>[2x]MHNDKDLSTWQTFRRLWPTIAPFKAGLIVAGVALILNAASDTFMLSLLKPLLDDGFGKTDRSVLVWMPLVVIGLMILRGITSYVSSYCISWVSGKVVMTMRRRLFGHMMGMPVSFFDKQSTGTLLSRITYDSEQVASSSSGALITVVREGASIIGLFIMMFYYSWQLSIILIVLAPIVSIAIRVVSKRFRNISKNMQNTMGQVTTSAEQMLKGHKEVLIFGGQEVETKRFDKVSNRMRLQGMKMVSASSISDPIIQLIASLALAFVLYAASFPSVMDSLTAGTITVVFSSMIALMRPLKSLTNVNAQFQRGMAACQTLFTILDSEQEKDEGKR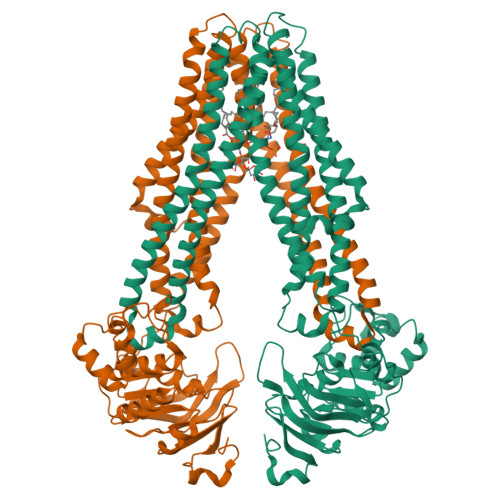VIERATGDVEFRNVTFTYPGRDVPALRNINLKIPAGKTVALVGRSGSGKSTIASLITRFYDIDEGEILMDGHDLREYTLASLRNQVALVSQNVHLFNDTVANNIAYARTEQYSREQIEEAARMAYAMDFINKMDNGLDTVIGENGVLLSGGQRQRIAIARALLRDSPILILDEATSALDTESERAIQAALDELQKNRTSLVIAHRLSTIEKADEIVVVEDGVIVERGTHNDLLEHRGVYAQLHKMQFGQ> MSHHHHHHKGLYFQQSSTDEEITFVFQEKEDLPVTEDNFVKLQVKACALSQINTKLLAEMKMKKDLFPVGREIAGIVLDVGSKVSFFQPDDEVVGILPLDSEDPGLCEVVRVHEHYLVHKPEKVTWTEAAGSIRDGVRAYTALHYLSHLSPGKSVLIMDGASAFGTIAIQLAHHRGAKVISTACSLEDKQCLERFRPPIARVIDVSNGKVHVAESCLEE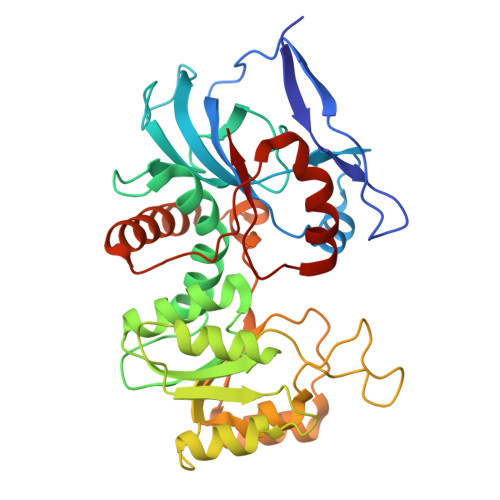TGGLGVDIVLDAGVRLYSKDDEPAVKLQLLPHKHDIITLLGVGGHWVTTEENLQLDPPDSHCLFLKGATLAFLNDEVWNLSNVQQGKYLCILKDVMEKLSTGVFRPQLDEPIPLYEAKVSMEAVQKNQGRKKQVVQF>[2x]SNAMLRWQTAGESHGEALVAMIEGLPAGVRISTDDIVSALARRRLGYGRGARMKFEQDKVRLLTGVRHGLTLGSP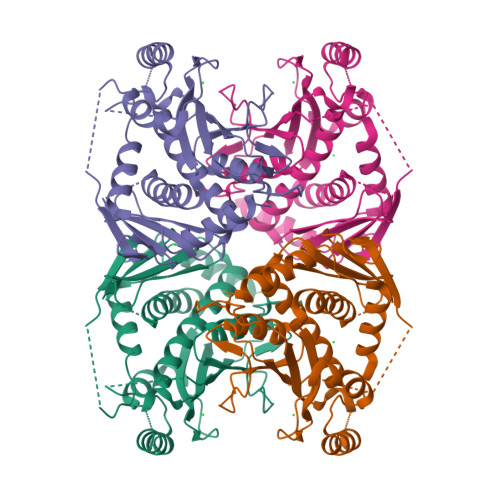VAIEIANTEWPKWTEVMSADALDHDLPREGRNAPLSRPRPGHADLTGMRKYGFDDARPVLERSSARETASRVALGEVAKQFLDQAFGIRTVAHVVALGGVQTNPDLPLPTPDDLEALDASPVRTLDKEAEVRIIERINEAKKAADTLGGVIEVLAYGVPAGIGTYVESDRRLDAALASAIMGIQAFKGVEIGDGFLAASRPGSQAHDEIVVNADGRIDRLSNRAGGIEGGMSNGQVIRVRGAMKPIPSIPKALRTVDVLTGESAQAINQRSDSTAVPAASVVAEAMVRLTLAKYALDKFGGDSVAETRRNLESYLASWPEHMR> MDLRVGRKFRIGRKIGSGSFGDIYHGTNLISGEEVAIRLESIRSRHPQLDYESRVYRYLSGGVGIPFIRWFGREGEYNAMVIDLLGPSLEDLFNYCHRRFSFKTVIMLALQMFCRIQYIHGRSFIHRDIKPDNFLMGVGRRGSTVHVIDFGLSKKYRDFNTHRHIPYRENKSLTGTARYASVNTHLGIEQSRRDDLESLGYVLIYFCKGSLPWQGLKATTKKQKYDRIMEKKLNVSVETLCSG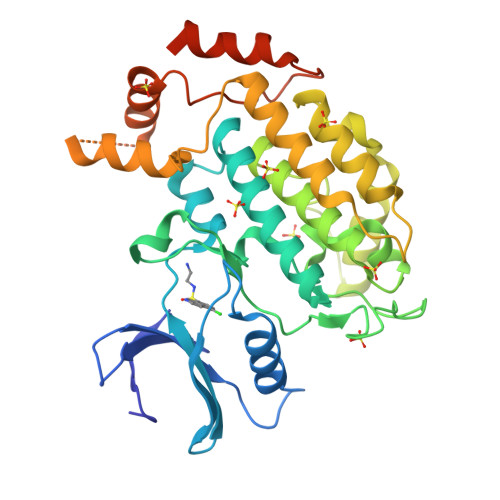LPLEFQEYMAYCKNLKFDEKPDYLFLARLFKDLSIKLEYHNDHLFDWTMLRYTKAMVEKQRDLLIEKGDLNANSNAASASNSTDNKSETFNKIKLLAMKKFPTHFHYYKNEDKHNPSPEEIKQQTILNNNAASSLPEELLNALDKGMENLR>[3x]LHQLSSPRYKFNFIADVVEKIAPAVVHIELFLRHPLFGRNVPLSSGSGFIMSEAGLIITNAHVVSSNSAAPGRQQLKVQLQNGDSYEATIKDIDKKSDIATIKIHPKKKLPVLLLGHSADLRPGEFVVAIGSPFALQNTVTTGIVSTAQREGRELGLRDSDMDYIQTDAIINYGNAGGPLVNLDGEVIGINTLKVTAGISFAIPSDRITRFLTEFQDKQIKDWKKRFIGIRMRTITPSLVDELKASNPDFPEVSSGIYVQEVAPNSPSQRGGIQDGDIIVKVNGRPLVDSSELQEAVLTESPLLLEVRRGNDDLLFSIAPEVVMGGHHHHHH

Human HtrA3, a proapoptotic protein, is a member of the HtrA (high temperature requirement A) family of homo-oligomeric serine proteases, which are well conserved in evolution and whose primary function is to maintain protein quality control. The long isoform of HtrA3 (HtrA3L) is a 49-kDa protein that contains a signal secretory peptide at the N-terminus (residues 1–17), a domain with homology to the insulin-like growth factor binding proteins (IGFBP) (residues 29–94) and a Kazal-type inhibitor motif (KI) (residues 89–126) followed by a serine protease domain (PD) with the catalytic triad H191-D227-S305 and one PDZ domain at the C-terminal end. HtrA3 is involved in the induction of the intrinsic, mitochondria-mediated apoptotic pathway. The common structural unit of the HtrA proteases is a pyramid-shaped trimer consisting of PDs, which form the central core, and outward-protruding PDZ domains.

The crystal structure of recombinant HtrA3 purified from bacterial cells containing two domains, PD and PDZ (ΔN-HtrA3S305A, residues 130–453), at a resolution of 3.27 Å was determined. The S305A mutation eliminated the serine protease activity causing partial degradation of the ΔN-HtrA3 protein and thus assured a high level of homogeneity for preparations. The asymmetric unit of the ΔN-HtrA3 crystals contains three molecules of the monomeric protein which represents the trimeric HtrA3 biological assembly. The trimer is stabilized by the interaction of three phenylalanines (F140, F142, and F255) from each monomer, forming a “lock” between monomers similar to other HtrA proteins. Two other chains encompass only PDs, residues 130–344 for chain B and 134–344 for chain C. Owing to the lack of electron density, the PDZ domains in the B and C chains are missing in the final structure, probably as a result of multiple domain positions inside the crystal. The ΔN-HtrA3 trimer structure appears to be in an intermediate conformation, lying between the flat saucer-like HtrA1 SAXS structure (“open form”) and the compact pyramidal HtrA2 X-ray structure (“closed form”). The main structural difference in ΔN-HtrA3 PD compared to the domain structures of HtrA1 and HtrA2 is the LB loop (residues 189–203), which is six residues longer than their counterparts. The interaction between the xxN-HtrA3 PD and PDZ domains through the unique extended LB loop, which carries the catalytic H191 residue, may be involved in HtrA3 activity regulation. The ΔN-HtrA3S305A active site is virtually the same as that observed in HtrA1S328A, with the catalytic serine residue (Ser305A) being too distant from His191 for proton transfer. Furthermore, the side-chain of L322 blocks access to the S1 specificity pocket similarly as L345 in the HtrA1 inactive PD (i.e., HtrA1_Cat(S328A) chain X).Spiroviolene synthase (SvS) from Streptomyces violens was first described by Rabe et al. and represents a bacterial class I diterpene cyclase that we were not able to produce in sufficient quantities for crystallization due to protein instability. Terpene cyclases such as SvS form a variety of complex multicyclic compounds with potent biological activities via carbocationic, electrophilic cyclization cascades of relatively simple substrates, either by metal-ion assisted release of an allylic pyrophosphate (class I mechanism) or by protonation of an oxirane/ene-functionality (class II mechanism). We previously reported a hypothetical ancestor of SvS—SvS-A2 26—which shares 77% sequence identity with the extant enzyme.

The variants could be grouped into four categories based on their substrate preference in a Malachite Green assay: promiscuous (I), inactive (II), diterpene-specific (III), or sesquiterpene-specific (IV). One representative variant of each group was subjected to crystal structure analysis, and Cα rmsd values in the range of 0.35–0.68 Å compared to the parental SvS-A2 structure indicated that none of the variants had significant conformational rearrangements. Furthermore, the studied variants were dimeric in the crystal structure and maintained a substantially elevated melting temperature similar to that of SvS-A2. The single residue exchange Ala224Ile (group IV) reverses substrate preference of the reconstructed ancestral enzyme and enhances specific activity for FPP approximately 3–5-fold (Malachite Green assay/GC-FID) compared to the reconstructed ancestral enzyme. Spiroviolene formation could not be detected for this variant so that a ratio of apparent second order rate constants cannot be derived. The isoleucine in this position is conserved in the two bacterial sesquiterpene cyclases SdS and HecS (Ile220 and Ile217, respectively),31,51 indicating that it may be a specificity switch of general importance in directing bacterial terpene cyclase sesquiterpene specificity. Changing this residue might affect metal binding as it is located upstream of the NSE motif. Steric effects are also likely to play a role, since the larger size of an isoleucine side chain permits sesquiterpene binding while hindering the correct positioning of the bulky diterpene substrate in the active site. In contrast, the Ala224Ile exchange slightly increases both the melting temperature of SvS-A2 (from 71.3 ± 0.0 °C to 73.4 ± 0.1 °C) and of SvS-WT (from 58.2 ± 0.1 °C to 63.6 ± 0.1 °C). The Ala224Ile exchange reverses substrate preference, and due to its conservation in a functionally related sesquiterpene cyclase, we speculate that it may represent a general specificity switch in bacterial terpene cyclases.

>MAMTVTEVDLPPIYCPLESAIHPRVHEVEKRAVEWIRRSGMCASEEERAWVIATHSADFFARFAPTAADEDRLLATSLWVYWGFAFDDHRCDNGPLSTRPAQFNALAGRVQRALEAPSAEDNGDRFVPALQDIARRFRSFGTPTQVRRFVHAHRAWLSGVAWQIGNQARGHMPGLDDYLAMRLLSAGGEPTFAMLEIATGAEVPDREMHRPAVRALTEMAIMVIALDNDRHSLRKELSRGHTDQNIYSVLMHHRGMSLQEAVEEATKLRDRILLRFLELHDRVRPGAGAELSTYLQGLRHGIRGNAEWGLRVPRYLSLGRVPDPMEDAPLTWAESPSDSSPSPLPGAPSIAWWWDDALLGA[2x]Human β1,3-galactosyltransferase 5 (β3GalT5) is a key enzyme involved in the synthesis of glycans on glycoproteins and glycolipids that are associated with various important biological functions, especially tumor malignancy and cancer progression, and has been considered as a promising target for development of anticancer agents. The catalytic domain adopts a mixed α/β Rossmann-like fold commonly observed in the GT-A glycosyltransferases superfamily and consists of a seven-stranded β sheet core (β1, β2, β3, β4, β5, β6, and β7) surrounded primarily by α helices (α1, α2, α3, α4, α5, α6, and α7), a two-strand antiparallel β sheet (β5′ and β7’),23 and an additional 13-residue α helix (α8) at the C terminus. Based on the structures obtained from our experiments, β3GalT5 catalyzes the transfer of galactose from UDP-Gal to a broad spectrum of glycan acceptors with an SN2-like mechanism; however, in the absence of a glycan acceptor, UDP-Gal is slowly converted to UDP and two other products, one is galactose through an SN2-like mechanism with water as an acceptor and the other is an oxocarbenium-like product, presumably through an SN1-like mechanisms. While β3GalT5 selectively binds to UDP-Gal as the donor substrate, it exhibits broader selectivity for acceptor substrates.

In total, we obtained eight structures, including β3GalT5 in complex with UDP-Gal, Gb4 glycan, GlcNac-β1,3-Gal, GlcNAc-β1,3-GalNAc, and Man-β1,6-Man. All structures belong to the P1 21 1 space group, with each asymmetric unit containing two protein molecules. Using disaccharides as substrates and measuring the end point UDP concentration after 1 h reaction time, we have selected Man-β1,6-Man and GlcNAc-β1,3-GalNAc-α-Thr in addition to Gb4 glycan and GlcNAc-β1,3-Gal-OMe for further structural studies of the enzyme–substrate complex obtained from β3GalT5 cocrystallized with UDP-Gal and soaked with various acceptors. The acceptor binding moiety has relatively fewer interactions in comparison to the donor binding moiety, resulting in a wider tolerance to different acceptors. The indole lid is turned off when no receptor is bound but is activated by forming a stacking interaction with the nonreducing end of acceptor.

>[2x]FKEQSFVYKKDGNFLKLPDTDCRQTPPFLVLLVTSSHKQLAERMAIRQTWGKERMVKGKQLKTFFLLGTTSSAAETKEVDQESQRHGDIIQKDFLDVYYNLTLKTMMGIEWVHRFCPQAAFVMKTDSDMFINVDYLTELLLKKNRTTRFFTGFLKLNEFPIRQPFSKWFVSKSEYPWDRYPPFCSGTGYVFSGDVASQVYNVSKSVPYIKLEDVFVGLCLERLNIRLEELHSQPTFFPGGLRFSVCLFRRIVACHFIKPRTLLDYWQALENSRGEDCP>[4x]MKQIKKLLVANRGEIAIRIFRAAAELDISTVAIYSNEDKSSLHRYKADESYLVGSDLGPAESYLNIERIIDVAKQANVDAIHPGYGFLSENEQFARRCAEEGIKFIGPHLEHLDMFGDKVKARTTAIKADLPVIPGTDGPIKSYELAKEFAEEAGFPLMIKATSGGGGKGMRIVREESELEDAFHRAKSEAEKSFGNSEVYIERYIDNPKHIEVQVIGDEHGNIVHLFERDCSVQRRHQKVVEVAPSVGLSPTLRQRICDAAIQLMENIKYVNAGTVEF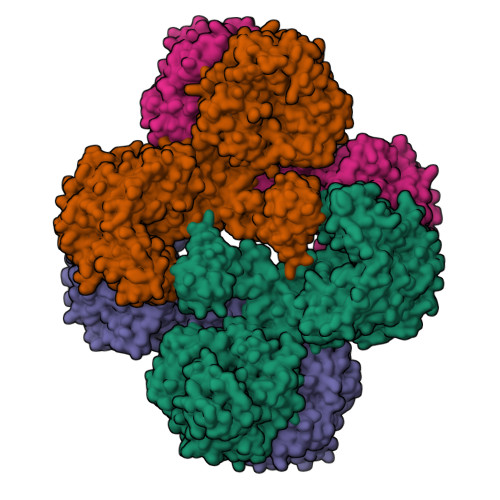LVSGDEFFFIEVNPRVQVEHTITEMVTGIDIVKTQILVAAGADLFGEEINMPQQKDITTLGYAIQCRITTEDPLNDFMPDTGTIIAYRSSGGFGVRLDAGDGFQGAEISPYYDSLLVKLSTHAISFKQAEEKMVRSLREMRIRGVKTNIPFLINVMKNKKFTSGDYTTKFIEETPELFDIQPSLDRGTKTLEYIGNVTINGFPNVEKRPKPDYELASIPTVSSSKIASFSGTKQLLDEVGPKGVAEWVKKQDDVLLTDTTFRDAHQSLLATRVRTKDMINIASKTADVFKDGFSLEMWGGTTFDVAYNFLKENPWERLERLRKAIPNVLFQMLLRASNAVGYKNYPDNVIHKFVQESAKAGIDVFRIFDSLNWVDQMKVANEAVQEAGKISEGTICYTGDILNPERSNIYTLEYYVKLAKELEREGFHILAIKDMAGLLKPKAAYELIGELKSAVDLPIHLHTHDTSGNGLLTYKQAIDAGVDIIDTAVASMSGLTSQPSANSLYYALNGFPRHLRTDIEGMESLSHYWSTVRTYYSDFESDIKSPNTEIYQHEMPGGQYSNLSQQAKSLGLGERFDEVKDMYRRVNFLFGDIVKVTPSSKVVGDMALYMVQNDLDEQSVITDGYKLDFPESVVSFFKGEIGQPVNGFNKDLQAVILKGQEALTARPGEYLEPVDFEKVRELLEEEQQGPVTEQDIISYVLYPKVYEQYIQTRNQYGNLSLLDTPTFFFGMRNGETVEIEIDKGKRLIIKLETISEPDENGNRTIYYAMNGQARRIYIKDENVHTNANVKPKADKSNPSHIGAQMPGSVTEVKVSVGETVKANQPLLITEAMKMETTIQAPFDGVIKQVTVNNGDTIATGDLLIEIEKATD>MGAPPLGPTIIPPVRTLWLRDRALDLDRVRLLGVLNLTPDSFSDGGRYLDPERALERAREMVAEGADILDLGAESTRPGAAPVPVEEEKRRLLPVLEAVLSLGVPVSVDTRKPEVAEEALKLGAHLLNDVTGLRDERMVALAARHGVAAVVMHMPVPDPATMMAHARYRDVVAEVKAFLEAQARRALSAGVPQVVLDPGFGFGKLLEHNLALLRRLDEIVALGHPVLVGLSRKRTIGELSGVEDPAQRVHGSVAAHLFAVMKGVRLLRVHDVRA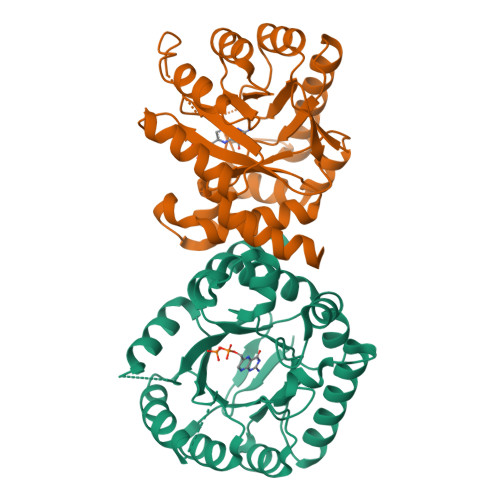HREALGVWEALYGGDRPSRA[2x]>[8x]MALDAFSKVVTNADAKAAYVGGADLQALKKFISEGNKRLDAVNSIVSNASCIVSDAVSGMICENPSLISPSGNCYTNRRMAACLRDGEIILRYVSYALLSGDSSVLEDRCLNGLKETYSSLGVPANSNARAVSIMKACAVAFVNNTASQRKLSTPQGDCSALASEVAGYFDKVSAAIG;>AFDKSAKAPVITIFDHRGCTAHKNAEYKGALTNSIDDEMCVKVQSV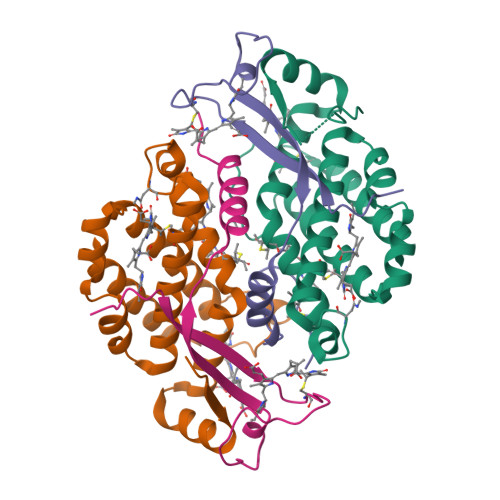KIAVSEADAAKKLQEFISYEAKGIDGAYTGRK[4x];>[4x]ADDKSGKAPVITVFDHRGCQRGGPDREYKGKKANGPDDEMCVKVQSAKIAVSATTADSVLQQTISTLYRK> AELVRTDSPNFLCSVLPSHWR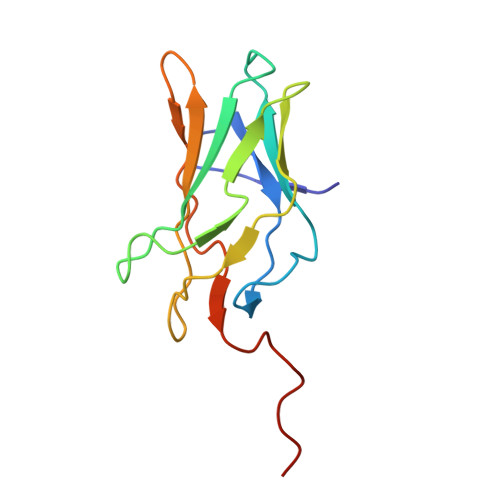CNKTLPVAFKVVALGEVPDGTVVTVMAGNDENYSAELRNASAVMKNQVARFNDLRFVGRSGRGKSFTLTITVFTNPPQVATYHRAIKVTVDGPREPRRHRQK>[2x]MCPILWTRNGSHCYYFSMEKKDWNSSLKFCADKGSHLLTFPDNQGVKLFGEYLGQDFY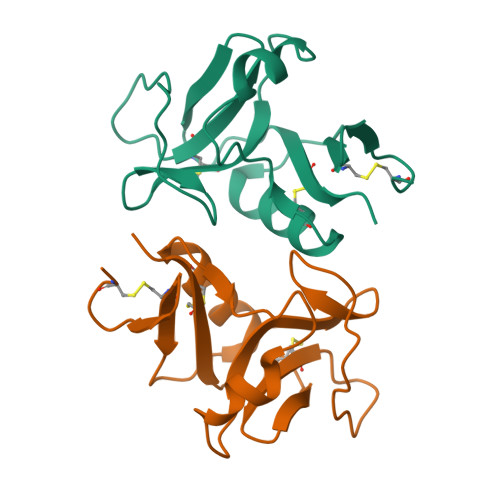WIGLRNIDGWRWEGGPALSLRILTNSLIQRCGAIHRNGLQASSCEVALQWICKKVLY> SMAFKRAIIFTSFNGFEKVSRTEKRRLAKIINARVSIIDEYLRAKDTNASLDGQYRAFLFNDESPAMTEFLAKLKAFAESCTGISIDAWEIEESEYVRLPVERRDFL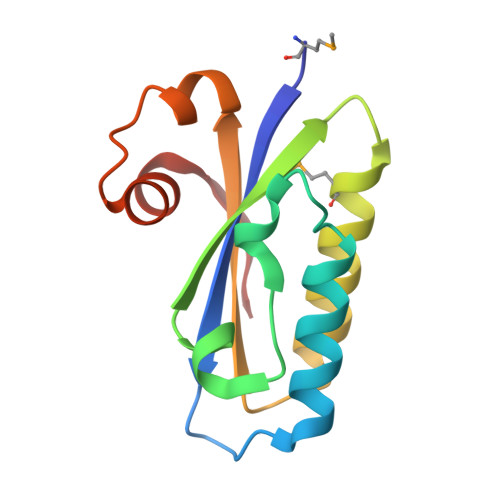AAANGKEIFKI> MKTEWPELVGKSVEEAKKVILQDKPA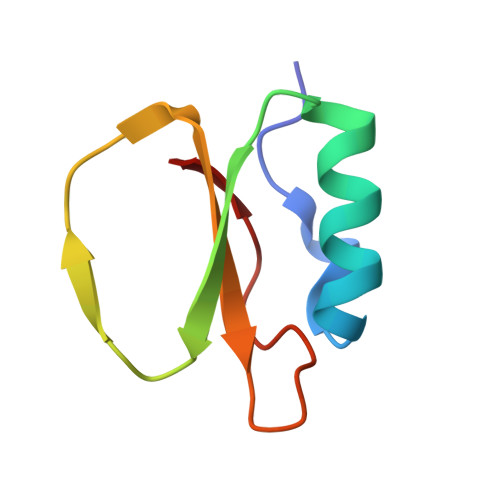AQIIVLPVGTIVTMEYRIDRVRLFVDRLDNIAQVPRVG ethyl 2-[4-(6-azanyl-5-cyano-pyrimidin-4-yl)pyrazol-1-yl]ethanoate | C12 H12 N6 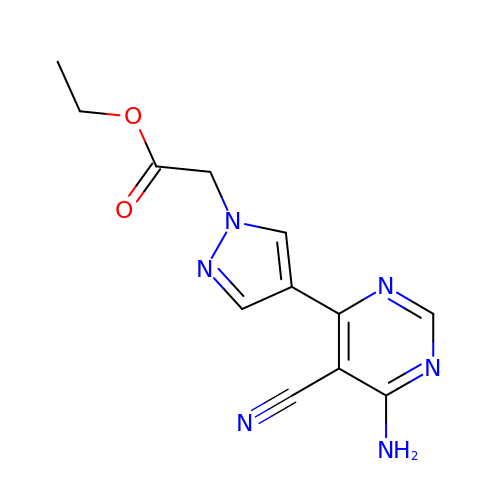O2 | PNBCCOMJHGKSBL-UHFFFAOYSA-N> KLGKLQYSLDYDFQNNQLLVGIIQAAELPALDMGGTSDPYVKVFLLPDKKKKFETKVHRKTLNPVFNEQFTFKVPYSELGGKTLVMAVYDFDRFSKHDIIGEFK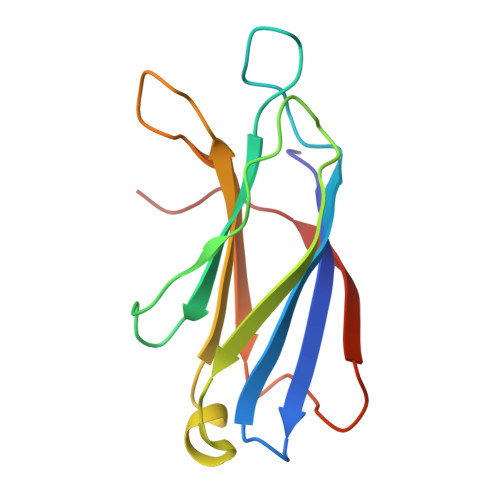VPMNTVDFGHVTEEWRDLQSAEK> ANSGEAPKNFGLDVKITGESENDRDLGTAPGGTLNDIGIDLRPWAFGQWGDWSAYFMGQAVAATDTIETDTLQSDTDDGNNSRNDGREPDKSYLAAREFWVDYAGLTAYPGEHLRFGRQRLREDSGQWQDTNIEALNWSFETTLLNAHAGVAQRFSEYRTDLDELAPEDKDRTHVFGDISTQWAPHHRIGVRIHHADDSGHLRRPGEEVDNLDKTYTGQLTWLGIEATGDAYNYRSSMPLNYWASATWLTGDRDNLTTTTVDDRRIATGKQSGDVNAFGVDLGLRWNIDEQWKAGVGYARGSGGGKDGEEQFQQTGLESNRSNFTGTRSRVHRFGEAFRGELSNLQAATLFGSWQLREDYDASLVYHKFWRVDDDSDIGTSGINAALQPGEKDIGQELDLVVTKYFKQGLLPASMSQYVDEPSALIRFRGGLFKPGDAYGPGTDSTMHRAFVDFIWRF

In the periplasm, M is randomly epimerized to G or partially acetylated, and the mature alginate is directed to the transmembrane β-barrel protein AlgE in the outer membrane for conveyance to the extracellular space. Briefly, the structures include 18 antiparallel strands (S1–S18) that cross the membrane to varying degrees, nine extracellular loops (L1–L9) and eight periplasmic turns (T1–T8). The loops and turns range in size from two to 43 residues, with L1 coordinating a calcium ion. Both the N- and C-termini are in the periplasm. The cavity within the AlgE barrel has been proposed to act as a pore for alginate, a random, linear copolymer of 1,4-linked β-d-mannuronic acid (M) and its C-5 epimer α-l-guluronic acid (G).

A number of different crystal forms were obtained, leading to several structures, the best having a resolution of 1.9 Å. The best crystals were obtained with 7.8 MAG at 20°C. These yielded three crystal forms in space groups C2, P212121, P21 that diffracted to 1.9, 2.4 and 2.8 Å resolution, respectively. AlgE-1.9 has one molecule in the asymmetric unit. In the AlgE-1.9 structure, electron density located toward the mid-membrane plane of the barrel and a little off-centre in the barrel cavity was well fitted by a citrate molecule. Citrate was present in the precipitant solution used for crystallization and is the likely source of the anion. It was not seen in the two other structures described in this study, in which T8 and L2 extend into the barrel with anionic side chains substituting, to some degree, for the bound citrate. We propose therefore that citrate acts as a mimic of the M and G components of alginate in AlgE-1.9. Further, its location within the 10 Å diameter electropositive pore serves to identify it as a limiting structure through which alginate passes in its transit across the protein and the outer membrane.>[2x]MKPNHLTLEQISLFKQLPGYWGCKDLNSVFVYANQAYGELIGLKRAEDCIGRTDFEMPSPTAACAAEFQQQDRYVIETGHSVKVLDIHPYPDGHWHAHIFTKTPWRDSQGK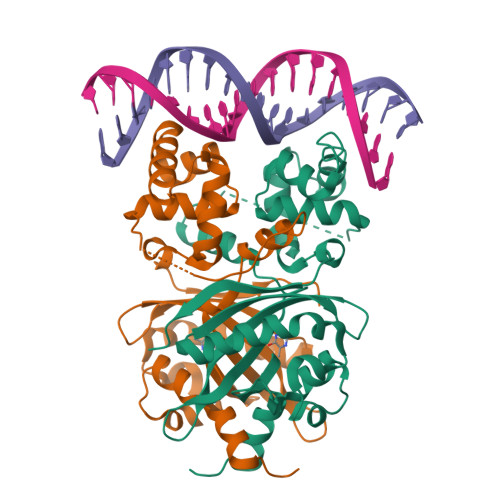IQGTIFFGQDLTDTAILEVGHWVCRATGLSTSTTFKSVADRDTLKLTARESEVLFLLLYGKKPQHIARVMGISIKTVEGYEAKLRSKFGALSKDQLIDLALDRGFGSVIPKTLLRKQLSVVLSDHTIPKKVDVVAQLLEHHHHHH[[(2R,3S,4R,5R)-5-(3-aminocarbonyl-4H-pyridin-1-yl)-3,4-bis(oxidanyl)oxolan-2-yl]methoxy-oxidanyl-phosphoryl] [(2R,3S,4R,5R)-5-(6-aminopurin-9-yl)-4-oxidanyl-3-phosphonooxy-oxolan-2-yl]methyl hydrogen phosphate | C21 H30 N7 O17 P3 | 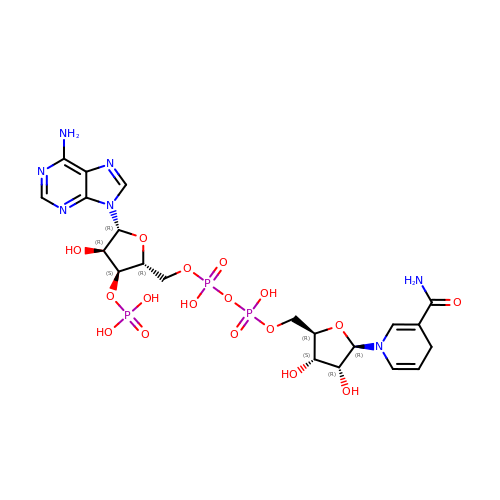ONOVTRNLNDQWGA-NNYOXOHSSA-N>SMNPVQLDDFDAYIKDMAKDSDYKFSLQFEELKLIGLDIPHFAADLPLNRCKNRYTNILPYDFSRVRLVSMNEEEGADYINANYIPGYNSPQEYIATQGPLPETRNDFWKMVLQQKSQIIVMLTQCNEKRRVKCDHYWPFTEEPIAYGDITVEMISEEEQDDWACRHFRINYADEMQDVMHFNYTAWPDHGVPTANAAESILQFVHMVRQQATKSKGPMIIHCSAGVGRT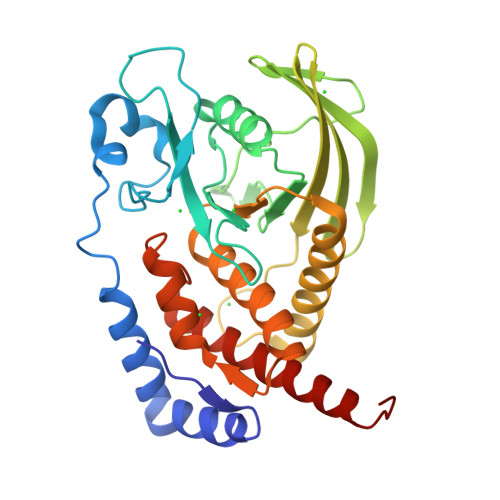GTFIALDRLLQHIRDHEFVDILGLVSEMRSYRMSMVQTEEQYIFIHQCVQLMWMKKKQQFCISDV[2x]> MILDVDYITEEGKPVIRLFKKENGKFKIEHDRTFRPYIYALLRDDSKIEEVKKITGERHGKIVRIVDVEKVEKKFLGKPITVWKLYLEHPQDVPTLREKVREHPAVVDIFEYDIPFAKRYLIDKGLIPMEGEEELKILAFDIETLYHEGEEFGKGPIIMISYADENEARVITWKNIDLPYVESVSTEKEMIKRFLRIIREKDPDIIVTYNGDSFDFPYLAKRAEKLGIKLTIGRDGSEPKMQRIGDMTAVEVKGRIHFDLYHVIRTTINLPTYTL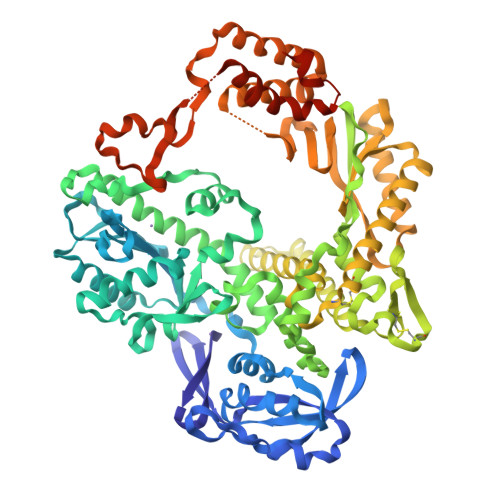EAVYEAIFGKPKEKVYADEIAKAWESGENLERVAKYSMEDAKATYELGKEFLPMEIQLSRLVGQPLWDVSRSSTGNLVEWFLLRKAYERNEVAPNKPSEEEYQRRLRESYTGGFVKEPEKGLWENIVYLDYKSLYPSIIITHNVSPDTLNLEGCKNYDIAPQVGHKFCKDIPGFIPSLLGHLLEERQKIKTKMKETQDPIEKILLDYRQKAIKLLANSFYGYYGYAKARWYCKECAESVTAWGRKYIELVWKELEEKFGFKVLYIDTDGLYATIPGGESEEIKKKALEFVKYINSKLPGLLELEYEGFYKRGFFVTKKRYAVIDEEGKVITRGLEIVRRDWSEIAKETQARVLETILKHGDVEEAVRIVKEVIQKLANYEIPPEKLAIYEQITRPLHEYKAIGPHVAVAKKLAAKGVKIKPGMVIGYIVLRGDGPISNRAILAEEYDPKKHKYDAEYYIENQVLPAVLRILEGFGYRKEDLRYQKTRQVGLTSWLNIKKS Introns of human transfer RNA precursors (pre-tRNAs) are excised by the tRNA splicing endonuclease TSEN in complex with the RNA kinase CLP1. The human TSEN complex consists of two catalytic subunits, TSEN2 and TSEN34, and two structural subunits, TSEN15 and TSEN54, all expressed at very low copy numbers of ~100 molecules per cell. In humans, TSEN2 and TSEN34 are each predicted to harbor a catalytic triad, composed of Tyr369/His377/Lys416 in TSEN2 and Tyr247/His255/Lys286 in TSEN34, responsible for cleavage at the 5′ and 3′ splice sites, respectively. Here, we show that intron excision is catalyzed by tetrameric TSEN assembled from inactive heterodimers independently of CLP1.

We re-cloned, co-expressed and purified the proteolytically characterized fragments, which readily formed rod-shaped crystals in space group P21 and diffracted X-rays to a resolution of 2.1 Å. The asymmetric unit is composed of two domain-swapped TSEN34 molecules, each binding one TSEN15 protomer at their C-terminal domains. The domain swap is brought about by a short, structured N-terminal α-helix/β-hairpin element of TSEN34 that is liberated to hook onto the neighboring protomer, presumably due to the truncated N-terminus of the molecule. The two TSEN15 and the two TSEN34 molecules in the asymmetric unit are very similar with average overall RMSDs of 0.37 and 0.50 Å, respectively. In one TSEN15 protomer, an elongated C-terminal region (residues 162–170) is visible, which is stabilized by crystal contacts. TSEN15 and TSEN34 display the typical endonuclease fold with the latter harboring the Tyr247/His255/Lys286 catalytic triad as also found in archaeal and eukaryotic endonucleases. In the interface between TSEN15 and TSEN34, two structural water molecules are found, which are coordinated by hydrogen bonds to backbone oxygens or amide groups of Ile110, Ala112, and Leu114 of TSEN15, Ile269, Leu271, and Gln272 of TSEN34, and the side-chain oxygen of Gln272. Furthermore, a YY motif in TSEN15 (Tyr152/Tyr153), which is conserved in eukaryotic endonucleases and archaeal α4- and (αβ)2-type endonucleases both stabilizes TSEN15 by hydrophobic interactions and the dimer interface by hydrogen bonds to the main-chain carbonyl oxygen of Leu274 and the side-chain oxygen of Ser283 of TSEN34. The imidazole group of His116 is central to a hydrogen bond network involving Asn117, Arg120, and Asp157 of TSEN15 and Ser292 and Thr302 of TSEN34. However, TSEN15 carrying the His-to-Tyr mutation engaged in complex formation with TSEN34 similar to the wt protein, and no impairment of catalytic activity was observed.

>[2x]MDWPHAGRPAHELRYSIYRDLWERGFFLSAAGKFGGDFLVYPGDPLRFHAHYIAQCWAPEDTIPLQDLVAAGRLGTSVRKTLLLCSPQPDGKVVYTSLQWASLQ;>MGHHHHHHHHHHGENLYFQGFGDGGGAPSWAPEDAWMGTHPKYLEMMELDIGDATQVYVAFLVYLDLMESKSWHEVNCVGLPELQLICLVGTEIEGEGLQTVVPTPITASLSHNRIREILKASRKLQGDPDLPMSFTLAIVESDSTIVYYKLTDGFMLPDPQNISLR[2x]>GSHMNITVSGDSSQLQSGMGLDKLIDGTTSSDDSSRMDLKWIFTSDQQDKGTLPFEMTFEFNEPKTLENFTIYNRMNSNGTINIAAMKKVKAVGYLNGEEFDLGEKANITSATTVYELGGKEFDKIVITALDSHKDKNTLAINEIEF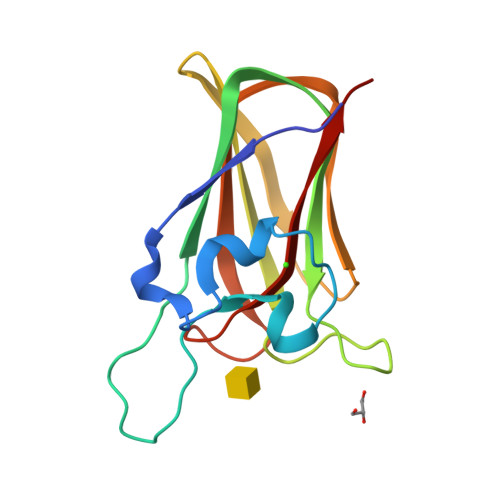YEKSE[2x]> LDFDILTNDGTHRNMKLLIDLKNIFSRQLPKMPKEYIVKLVFDRHHESMV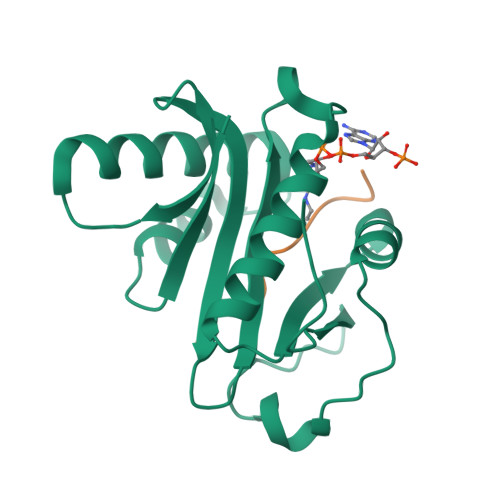ILKNKQKVIGGICFRQYKPQRFAEVAFLAVTANEQVRGYGTRLMNKFKDHMQKQNIEYLLTYADNFAIGYFKKQGFTKEHRMPQEKWKGYIKDYDGGTLMECYIHPYVDYGR;> KSTGGKAPRKQ>[2x]MAEKPKLHYFNARGRMESTRWLLAAAGVEFEEKFIKSAEDLDKLRNDGYLMF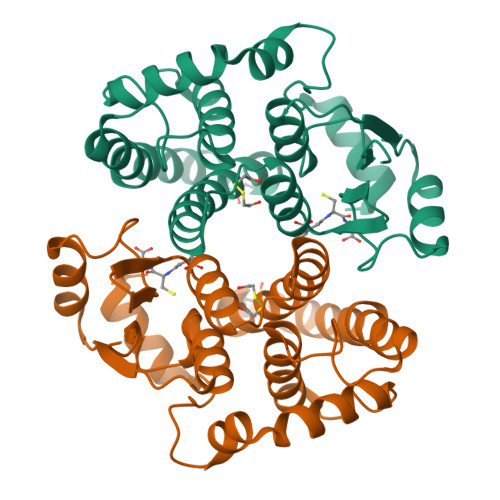QQVPMVEIDGMKLVQTRAILNYIASKYNLYGKDIKERALIDMYIEGIADLGEMILLLPVCPPEEKDAKLALIKEKIKNRYFPAFEKVLKSHGQDYLVGNKLSRADIHLVELLYYVEELDSSLISSFPLLKALKTRISNLPTVKKFLQPGSPRKPPMDEKSLEEARKIFRF>ETFTVKMGADSGLFQFEPANVTVHPGDTVKWVNNKLPPHNILFDDKQVPGASKELADKLSHSQLMFSP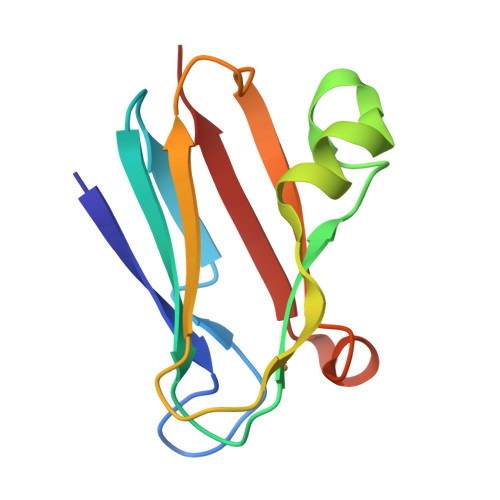GESYEITFSSDFPAGTYTYYCAPHRGAGMVGKITVEG[2x]>AECSVDIQGNDQMQFNTNAITVDKSCKQFTVNLSHPGNLPKNVMGHNWVLSTAADMQGVVTDGMASGLDKDYLKPDDSRVIAHTKLIGSGEKDS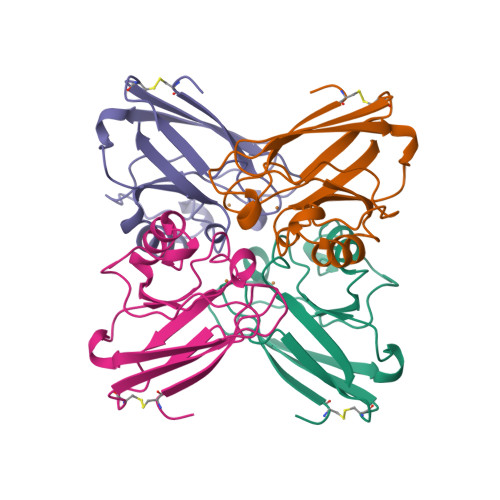VTFDVSKLKEGEQYMFFCTFPGHSALAKGTLTLK[4x]>[2x]MESTTEVTGATGVVTNVAAAPLPEATSSMSLAPTVNSIDPWIFLNPTEVPGGTFTVASNTQPGTMLLDIEISPELNIFTAHMFRMYAGWSGGFAIKLLVAGNAFSAGKLIVAIIPPNVQVPNSAYLLTGFPHEILDFRTADQVEIIAPDIKNLDYHFRGDKLGRLVVMVYSPLRSTATDFEIEIKLLSAPLPDFKFTMLVPPVQNNALPIWQIPPTPPGAMVNPRSPLTPVVDLYINSSWTTCNHQLGRYTIDGGAIGNSTFNPSGLWTGTFTAESGSVSGQTNWRIAMLDN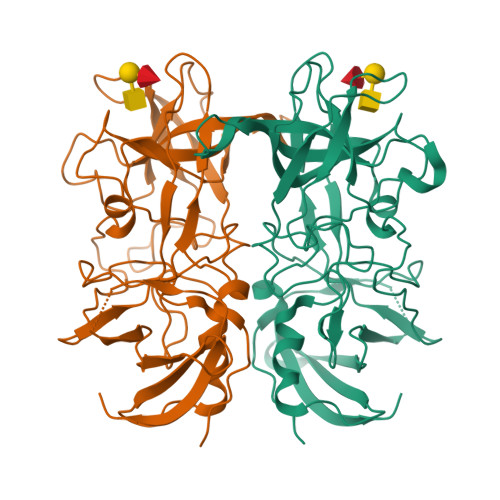PYNPTSDPTLPPVPRGFCDWGSGVKSGARQHLVCFTGVETDNGEGYKDVDAHMWDYGDDATIGLDNTYQRQIYISDPTALDSGKRYIIIPMGASGSATDDTLQISPNCYGSWDYAPTIAPPLGEQIVWFRSYLPASSTSASSGVNSVSAHISSLMSPDLIRSAYVSGFPEGKAALLDYVLYGGSVVEQFKMYREGYLTANATGTNTGFIIPPDGYFRFNSWVSPTFVIGNVVDLSSSRSLTFH> GSHMVPDTPTRLVFSALGPTSLRVSWQEPRCERPLQGYSVEYQLLNGGELHRLNIPNPAQTSVVVEDLLPNHSYVFRVRAQSQEGWGREREGVITIESQVHPQSPLCPLPGSAFTLSTPSAPGP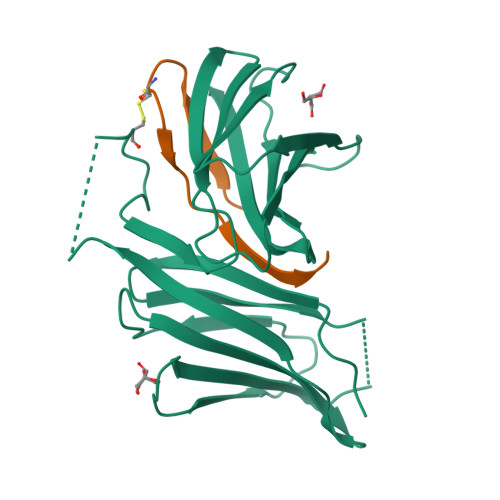LVFTALSPDSLQLSWERPRRPNGDIVGYLVTCEMAQGGGPATAFRVDGDSPESRLTVPGLSENVPYKFKVQARTTEGFGPEREGIIRIES;> DSNENLLLVHCGPTLINSCISFGSESFDGH5'-O-[(R)-(butylamino)(hydroxy)phosphoryl]adenosine | C14 H23 N6 O6 P | 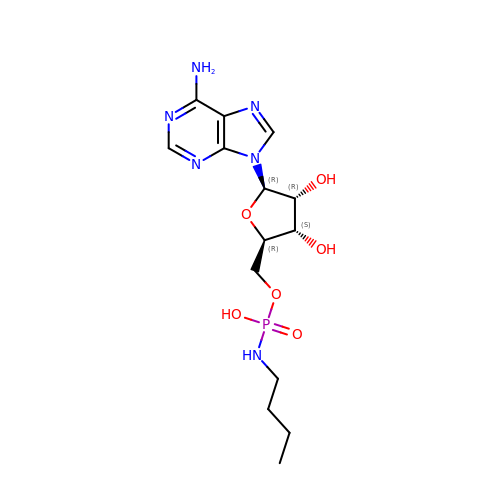JCDWYZKYCCUIPS-IDTAVKCVSA-N> STDNAETGVIEAGNTDTDFSGELAAPGSNHTNVKFLFDRSRLLNVIKVLEKDAVFPRPFPTATGTQQDDGYFCLLTPRPTVASRPATRFGLYVSPSDSGVLANTSLDFNFYSLACFTYFRSDLEVTVVSLEPDLEFAVGWFPSGSEYQASSFVYDQLHVPYHFTGRTPRAFASKGGKVSFVLPWNSVSSVLPVRWGGASKLSSATRGLPAHADWGTIYAFIPRPNEKKST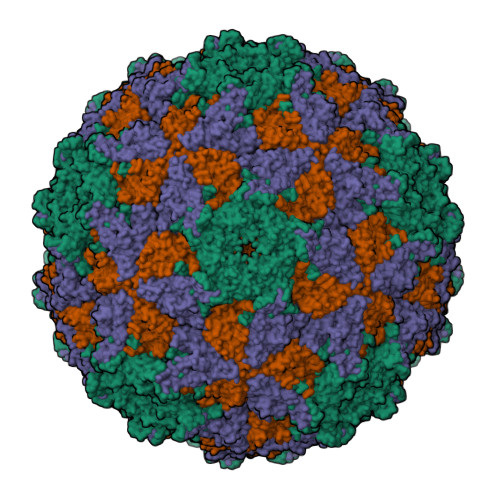AVKHVAVYIRYKNARAWCPSMLPFRSYK;> DRVTTQTAGNTAINTQSSLGVLCAYVEDPTKSDPPSSSTDQPTTTFTAIDRWYTGRLNSWTKAVKTFSFQAVPLPGAFLSRQGGLNGGAFTATLHRHFLMKCGWQVQVQCNLTQFHQGALLVAMVPETTLDVKPDGKAKSLQELNEEQWVEMSDDYRTGKNMPFQSLGTYYRPPNWTWGPNFINPYQVTVFPHQILNARTSTSVDINVPYIGETPTQSSETQNSWTLLVMVLVPLDYKEGATTDPEITFSVRPTSPYFNGLRNRYTT;> GPIPTAPRENSLMFLSTTPDDTVPAYGNVRTPPVNYLPGEITDLLQLARIPTLMAFGRVPEPEPASDAYVPYVAVPTQFDDKPLISFPITLSDPVYQNTLVGAISSNFANYRGCIQITLTFCGPMMARGKFLLSYSPPNGTQPQTLSEAMQCTYSIWDIGLNSSWTFVIPYISPSDYRETRAITNSVYSADGWFSLHKLTKITLPPDCPQSPCILFFASAGEDYTLRLPVDCNPSYVFH;> GNVQTTSKNDFDSRGNNGNMTFNYYANTYQNSVDFSTSSSASGAGPGNSRGGLAGLLTNFSGILNPLGYLK> GI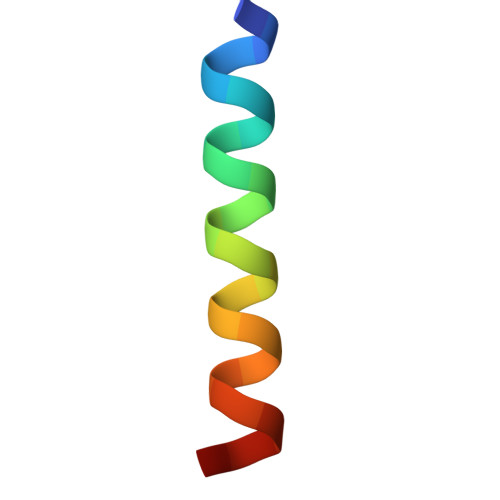GKFLHAAKKFAKAFVAEIMNS(9Z,11E,13S)-13-hydroxyoctadeca-9,11-dienoic 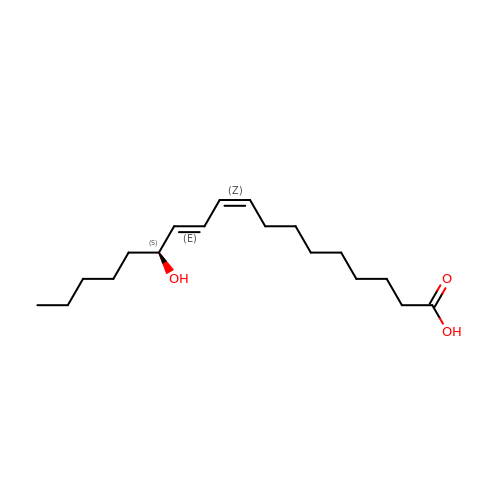acid | C18 H32 O3 | HNICUWMFWZBIFP-IRQZEAMPSA-N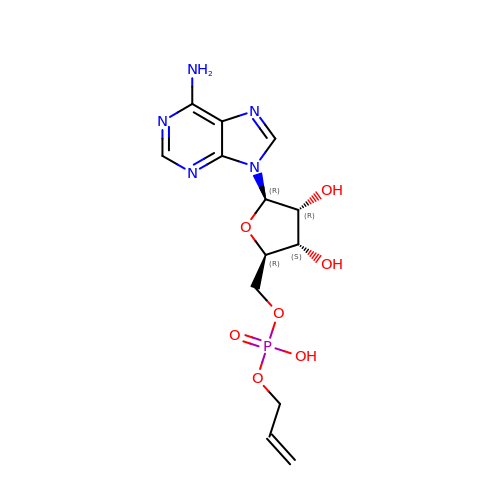5'-O-{(S)-hydroxy[(prop-2-en-1-yl)oxy]phosphoryl}adenosine | C13 H18 N5 O7 P | LNGYCTNQUWBENP-QYVSTXNMSA-N> MEVKKFKRFESYKRDNQLPPKVRDMGIVIDQKNNTIVLPIMG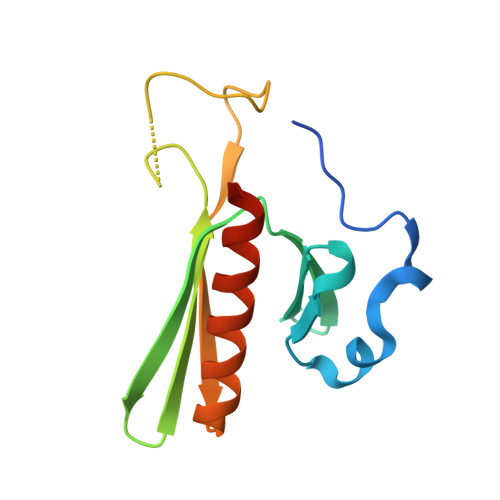RPVPFHINTIKNASKSDEGEWSFLRINFLSPGQGVGRKDDQPFEDASAHFVRSLTFRSTDGDRYAEIANQISNLKREAVKREQEK> STWIENKLYGM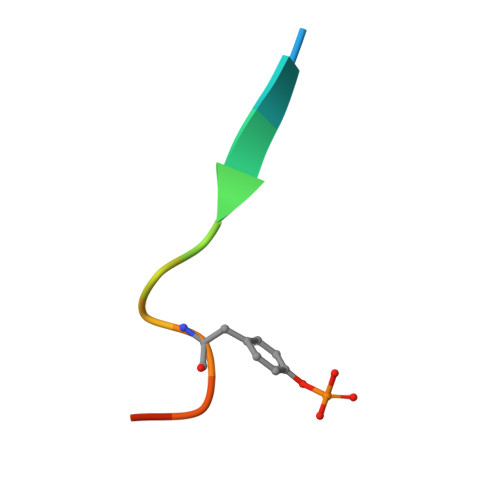SD(2R)-2-(2-fluorophenyl)-3-[2-[4-[(2R)-2-(2-fluorophenyl)-4-oxidanylidene-1,2-dihydroquinazolin-3-yl]piperidin-1-yl]ethyl]-1,2-dihydroquinazolin-4-one | C35 H33 F2 N5 O2 | 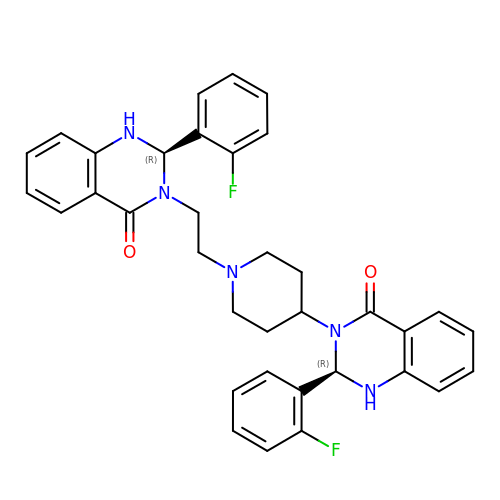ZMXNWFRGUZJFLG-CZNDPXEESA-N> MAKKTSSRQRRPWEPPLDKGTVPWLGHAMAFRKNMFEFLKRMRTKHGDVFTVQLGGQYFTFVMDPLSFGSILKDTQRKLDFGQYAKKLVLKVFGYRSVQGDHEMIH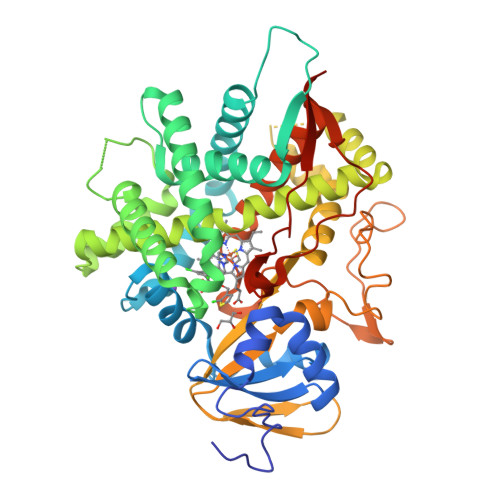SASTKHLRGDGLKDLNETMLDSLSFVMLTSKGWSLDASCWHEDSLFRFCYYILFTAGYLSLFGYTKDKEQDLLQAGELFMEFRKFDLLFPRFVYSLLWPREWLEVGRLQRLFHKMLSVSHSQEKEGISNWLGNMLQFLREQGVPSAMQDKFNFMMLWASQGNTGPTSFWALLYLLKHPEAIRAVREEATQVLGEARLETKQSFAFKLGALQHTPVLDSVVEETLRLRAAPTLLRLVHEDYTLKMSSGQEYLFRHGDILALFPYLSVHMDPDIHPEPTVFKYDRFLNPNGSRKVDFFKTGKKIHHYTMPWGSGVSICPGRFFALSEVKLFILLMVTHFDLELVDPDTPLPHVDPQRWGFGTMQPSHDVRFRYRLHPTEHHHHHH> MESKVVVPAQGKKITLQNGKLNVPENPIIPYIEGDGIGVDVTPAMLKVVDAAVEKAYKGERKISWMEIYTGEKSTQVYGQDVWLPAETLDLIREYRVAIKGPLTTPVGGGIRELNVALRQELDLYICLRPVRYYQGTPSPVKHPELTDMVIFRENSEDIYAGIEWKADSADAEKVIKFLREEMGVKKIRFP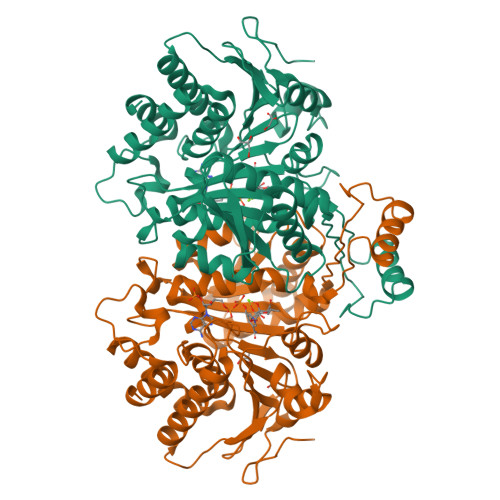EHCGIGIKPCSEEGTKRLVRAAIEYAIANDRDSVTLVHKGNIMKFTEGAFKDWGYQLAREEFGGELIDGGPWLKVKNPNTGKEIVIKDVIADAFLQQILLRPAEYDVIACMNLNGDYISDALAAQVGGIGIAPGANIGDECALFEATHGTAPKYAGQDKVNPGSIILSAEMMLRHMGWTEAADLIVKGMEGAINAKTVTYDFERLMDGAKLLKCSEFGDAIIENM3-[2-[(Z)-[3-(2-carboxyethyl)-5-[(Z)-(4-ethenyl-3-methyl-5-oxidanylidene-pyrrol-2-ylidene)methyl]-4-methyl-pyrrol-1-ium-2-ylidene]methyl]-5-[(Z)-[(3E)-3-ethylidene-4-methyl-5-oxidanylidene-pyrrolidin-2-ylidene]methyl]-4-methyl-1H-pyrrol-3-yl]propanoic 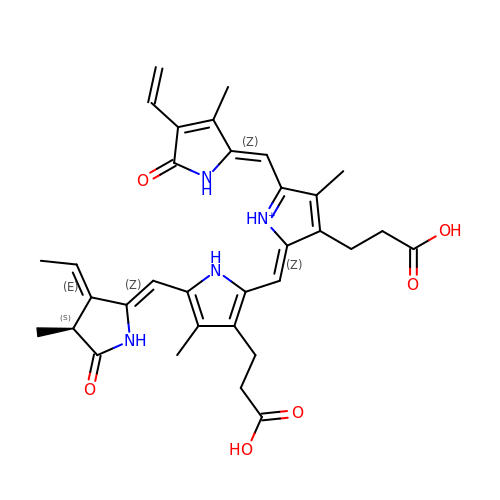acid | C33 H37 N4 O6 | DKMLMZVDTGOEGU-ISEYCTJISA-O> GPDSMLADSFEQEASREVDASKGLTNSETLQVEQDGKVRLSHQVRHQVALPPNYDYTPIAEHKRVNEARTYPFTLDPFQDTAISCIDRGESVLVSAHTSAGKTVVAEYAIAQSLKNKQRVIYTSPIKALSNQKYRELLAEFGDVGLMTGDITINPDAGCLVMTTEILRSMLYRGSEVMREVAWVIFDEVHYMRDKERGVVWEETIILLPDKVRYVFLSATIPNAMEFAEWICKIHSQPCHIVYTNFRPTPLQHYLFPAHGDGIYLVVDEKSTFREENFQKAMASISNQIGDDPNSTDSRGKKGQTYKGGSAKGDAKGDIYKIVKMIWKK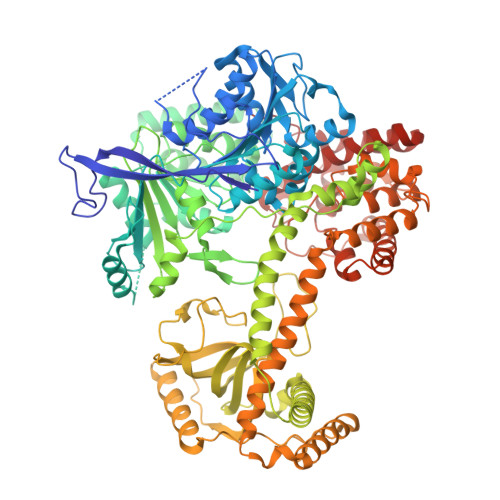KYNPVIVFSFSKRDCEELALKMSKLDFNSDDEKEALTKIFNNAIALLPETDRELPQIKHILPLLRRGIGIHHSGLLPILKEVIEILFQEGFLKVLFATETFSIGLNMPAKTVVFTSVRKWDGQQFRWVSGGEYIQMSGRAGRRGLDDRGIVIMMIDEKMEPQVAKGMVKGQADRLDSAFHLGYNMILNLMRVEGISPEFMLEHSFFQFQNVISVPVMEKKLAELKKDFDGIEVEDEENVKEYHEIEQAIKGYREDVRQVVTHPANALSFLQPGRLVEISVNGKDNYGWGAVVDFAKRINKRNPSAVYTDHESYIVNVVVNTMYIDSPVNLLKPFNPTLPEGIRPAEEGEKSICAVIPITLDSIKSIGNLRLYMPKDIRASGQKETVGKSLREVNRRFPDGIPVLDPVKNMKIEDEDFLKLMKKIDVLNTKLSSNPLTNSMRLEELYGKYSRKHDLHEDMKQLKRKISESQAVIQLDDLRRRKRVLRRLGFCTPNDIIELKGRVACEISSGDELLLTELIFNGNFNELKPEQAAALLSCFAFQERCKEAPRLKPELAEPLKAMREIAAKIAKIMKDSKIEVVEKDYVESFRHELMEVVYEWCRGATFTQICKMTDVYEGSLIRMFKRLEELVKELVDVANTIGNSSLKEKMEAVLKLIHRDIVSAGSLYL> SNAAGFAQASPSAPVAGKDFEVMKSPQPVSAPAGKVEVIEFFWYGCPHCYEFEPTIEAWVKKQGDKIAFKRVPVAFRDDFVPHSKLFYALAALGV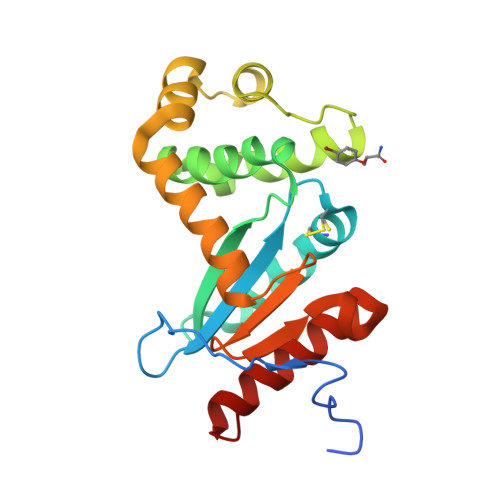SEKVTPAVFNAIHKEKNYLLTPQAQADFLATQGVDKKKFLDAYNSFSVQGQVKQSAELLKNYNIDGVPTIVVQGKYKTGPAYTNSLEGTAQVLDFLVKQVQDKKL> MRKMAVISLVLLLFLVGCGKEEAAQKPEQKTDKEPKIVATTVAITEIMDKLDLPLVGIPSSSKKLPKRYADVKETGSPMGPDLEIIRMLKPDMVLSTKTLEADLKSGFEGADLEADFLDFTSIASMQTEIKNLGAKFDRIEEATKLNKDLTSDIDQVKSNVAKKKKPTVLILMGVPGSYLVVTEHAYIGDLVKLAGGENVIKDQKVEYLASNTEYLQSANPDIILR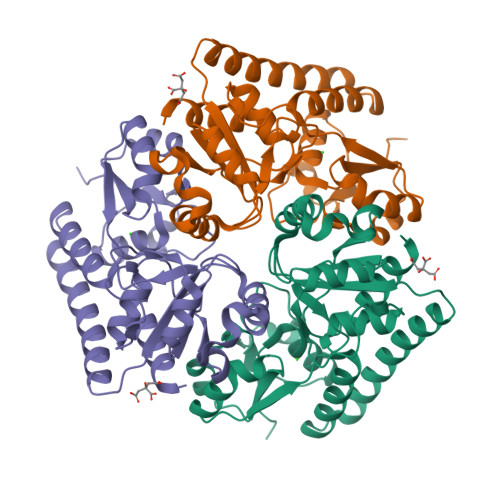AAHGMPAEVVKMFDEEFKTNDIWKHFDAVKNNRVYDLDENLFGMTASLNAPEALKEMEKMLYDN> GGGUACUUAAGCCCACUGAUGAGUCGCUGGGAUGCGACAAAACGCCCA;> GGGCGUCUGGGCA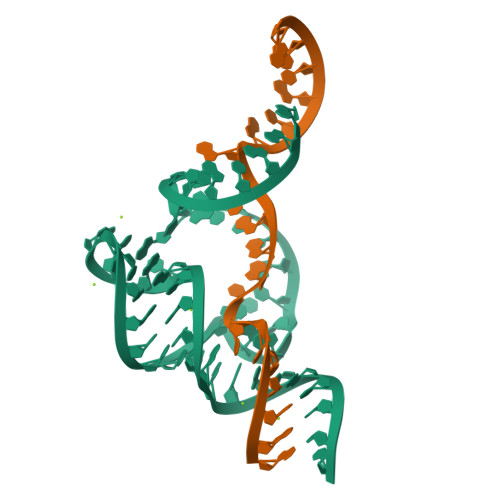GUACCCA>EPAFNYAEALQKSMFFYEAQRSGKLPENNRVSWRGDSGLNDGADVGLDLTGGWYDAGDHVKFGFPMAFTATMLAWGAIESPEGYIRSGQMPYLKDNLRWVNDYFIKAHPSPNVLYVQVGDGDADHKWWGPAEVMPMERPSFKVDPSCPGSDVAAETAAAMAASSIVFADDDPAYAATLVQHAKQLYTFADTYRGVYSDCVPAGAFYNSWSGYQDELVWGAYWLYKATGDDSYLAKAEYEYDFLSTEQQTDLRSYRWTIAWDDKSYGTYVLLAKETGKQKYIDDANRWLDYWTVGVNGQRVPYSPGGMAVLDTWGALRYAANTAFVALVYAKVIDDPVRKQRYHDFAVRQINYALGDNPRNSSYVVGFGNNPPRNPHHRTAHGSWTDSIASPAENRHVLYGALVGGPGSPNDAYTDDRQDYVANEVATDYNAGFSSALAMLVEEYGGTPLADFPPTEEPDGPEIFVEAQINTPGTTFTEIKAMIRNQSGWPARMLDKGTFRYWFTLDEGVDPADITVSSAYNQCATPEDVHHVSGDLYYVEIDCTGEKIFPGGQSEHRREVQFRIAGGPGWDPSNDWSFQGIGNELAPAPYIVLYDDGVPVWGTAP[2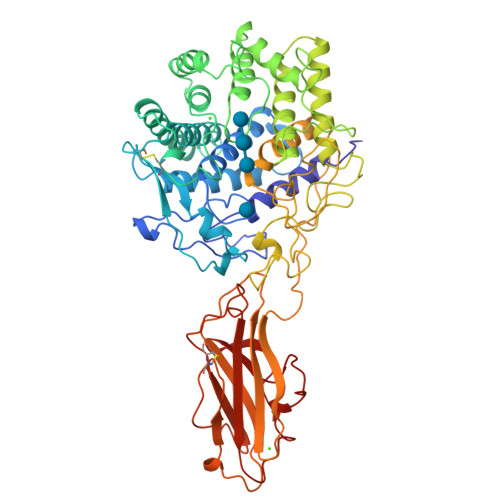x]>[4x]HHHHHHSSGLVPRGSHMLRRTSSTFSAKRVFVVGGHITTFVGKGSPLFIDKKHPDFGKKENKTLEELLAESINGALQNTGLHDGRAALVDKLVVGNFL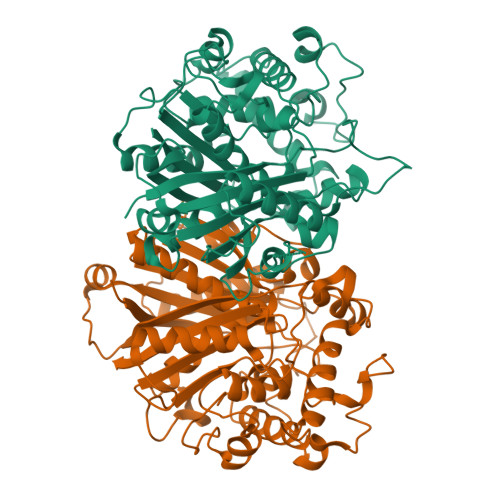GELFSSQGHLGPAAVGSLSGSNSSAFLNKPAVRVEGACASGGLAVQSAWEALLAGTSQIALAVGVEVQTTVSARVGGDYLARAAHYKRQRQLDDFTFPCLFARRMKAIQEAGHFTMEDAAYVAAKAYASGNRNPLAHMHARKVTLDFCTQASDKNPNFLGNEIYKPFLRTTDCSQVSDGGAAVILASEEGLQKLGLSPNDNRLVEIKSLASAAGNLYEDSPDLTRMTTSMVAARTALSMAGVKPEQLQVAEVHDCFTIAELLMYEALGIAEYGGAGALIRSGATALDGRIPVNTGGGLLSFGHPVGATGVKQVLEVYRQMKGQCGEYQMKNIPGIGATLNMGGDDKTAVSMVLTNI> QFRAIIESPEGAGHVGYQYRRNTGSTMRMVSDVLDERVSLWDFHCDPSGNVIQPGPNVDSRQYLQAAIDYVSSNGGGTITIPAGYTWYLGSYGVGGIAGHSGIIQLRSNVNLNIEGRIHLSPFFDLKPFQVFVGFDNGDPASSGNLENCHIYGHGVVDFGGYEFGASSQLRNGVAFGRSYNCSVTGITFQNGDVTWAITLGWNGYGSNCYVRKCRFINLVNSSVNANHSTVYVNCPYSGVESCYFSMSSSFARNIACSVQLHQHDTFYRGSTVNGYCRGAYVVMHAAEAAGAGSYAYNMQVENNIAVIYGQFVILGSDVTATVSGHLNDVIVSGNIVSIGERAAFSAPFGAFIDIGPDNSGASNVQDIQRVLVTGN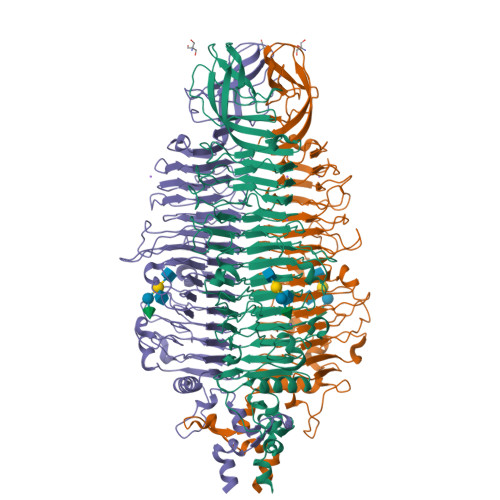SFYAPANITDSAAITLRANLNGCTFIANNFDCRYMVYNAPGTTSPVVQNLVWDKSNVIGGTHANQRAGQNLFDMQFASVVNSTIEVQLSCEDLSMFSCILFPASCQLSYSKITVDSAWTKSMSNTAVFEGNQQAGANVYVSYPATVNLTSYNTQGAVPFFSTDTNYAWVTSAYSLSINENLDFSPPATYTNKANGQLVGVGYNEIGGVRSVSVRLMLQRQV>MAQIDFRKKINWHRRYRSPQGVKTEHEILRIFESDRGRIINSPAIRRLQQKTQVFPLERNAAVRTRLTHSMEVQQVGRYIAKEILSRLKELKLLEAYGLDELTGPFESIVEMSCLMHDIGNPPFGHFGEAAINDWFRQRLHPEDAESQPLTDDRCSVAALRLRDGEEPLNELRRKIRQDLCHFEGNAQGIRLVHTLMRMNLTWAQVGGILKYTRPAWWRGETPETHHYLMKKPGYYLSEEAYIARLRKELNLALYSRFPLTWIMEAADDISYCVADLEDAVEKRIFTVEQLYHHLHEAWGQHEKGSLFSLVVENAWEKSRSNSLSRSTEDQFFMYLRVNTLNKLVPYAAQRFIDNLPAIFAGTFNHALLEDASECSDLLKLYKNVAVKHVFSHPDVERLELQGYRVISGLLEIYRPLLSLSLSDFTELVEKERVKRFPIESRLFHKLSTRHRLAYVEAVSKLPSDSP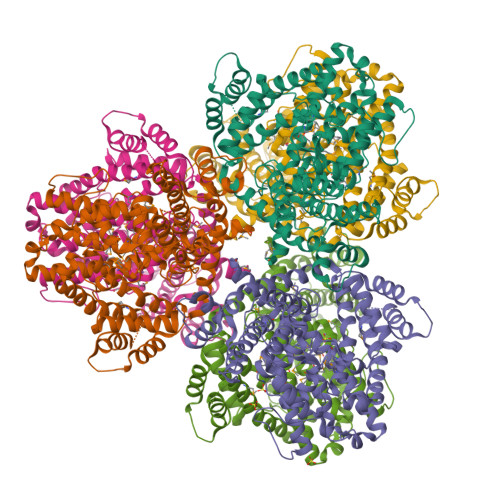EFPLWEYYYRCRLLQDYISGMTDLYAWDEYRRLMAVEQ[6x]> MTPPLATTIDRLRDYLDRVG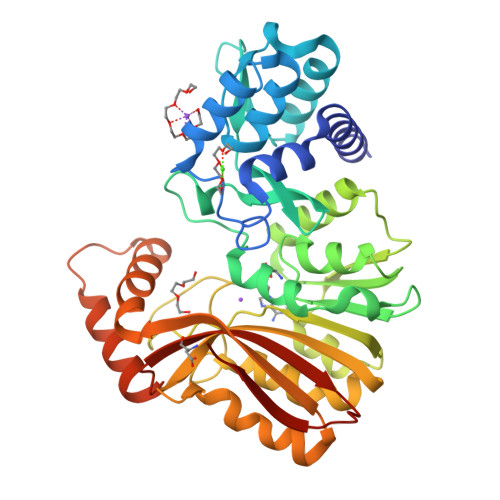FQQIYKYIVAVNHYAVTPALITRNTAASVHHFFDSRLGGRAEFALLQCLMTGRPAEHAALPDKDRALADALVTAGLLRASPDGREVSGADRQLISAFGVDLLIDRRIHFGGEVHEVFIGPDSYWMLYYINASGIARTHRAVDLCTGSGIAALYLSLFTDHVLATDIGDVPLALVEINRRLNRRDAGTMEIRRENLNDTLDGRERFDLLTCNPPFVAFPPGYSGTLYSQGTGVDGLGYMRDIVGRLPEVLNPGGSAYLVADLCGDAHGPHFLGELESMVTGHGMRIEAFIDHVLPASAQVGPISDFLRHAAGLPADTDIAADVQAFQRETLRADYYYLTTIRLQTAAQNPGLRMLRRDPLPGAGT>G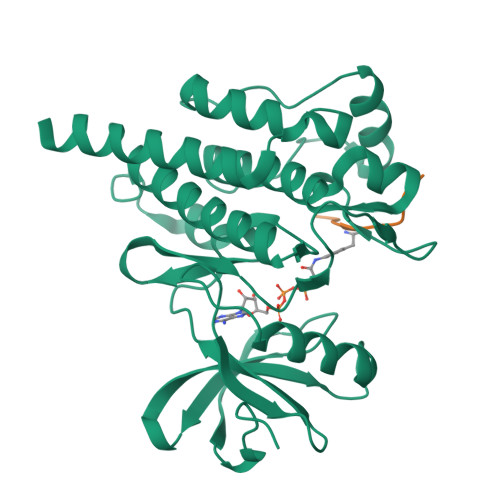HMSPNYDKWEMERTDITMKHKLGGGQYGEVYEGVWKKYSLTVAVKTLKEDTMEVEEFLKEAAVMKEIKHPNLVQLLGVCTREPPFYIITEFMTYGNLLDYLRECNRQEVNAVVLLYMATQISSAMEYLEKKNFIHRDLAARNCLVGENHLVKVADFGLSRLMTGDTYTAPAGAKFPIKWTAPESLAYNKFSIKSDVWAFGVLLWEIATYGMSPYPGIDLSQVYELLEKDYRMERPEGCPEKVYELMRACWQWNPSDRPSFAEIHQAFETMFQESSISDEVEKELGK[2x];> EAIFAAPFAKK>APASLLPPAPEHSPPSSPLTQPPEGPKFPRVKNWEVGSITYDTLSAQAQQDGPCTPRRCLGSLVFPRKLQGRPSPGPPAPEQLLSQARDFINQYYSSIKRSGSQAHEQRLQEVEAEVAATGTYQLRESELVFGAKQAWRNAPRCVGRIQWGKLQVFDARDCRSAQEMFTYICNHIKYATNRGNLRSAITVFPQRCPGRGDFRIWNSQLVRYAGYRQQDGSVRGDPANVEITELCIQHGWTPGNGRFDVLPLLLQAPDEPPELFLLPPELVLEVPLEHPTLEWFAALGLRWYALPAVSNMLLEIGG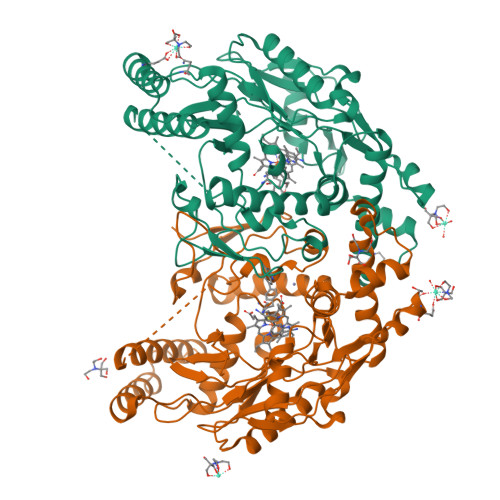LEFPAAPFSGWYMSTEIGTRNLCDPHRYNILEDVAVCMDLDTRTTSSLWKDKAAVEINVAVLHSYQLAKVTIVDHHAATASFMKHLENEQKARGGCPADWAWIVPPISGSLTPVFHQEMVNYFLSPAFRYQPDPW[6x]HPRT is a purine salvage enzyme that converts purine bases and PRPP to GMP and IMP, which are precursors of the essential nucleotide GTP. HPRT activity was previously found to be inhibited by (p)ppGpp in several bacteria including Bacillus subtilis. To examine the molecular determinants underlying (p)ppGpp regulation of HPRT, we turned to Hpt-1 from the pathogenic bacterium B. anthracis, which pppGpp competitively inhibits similarly to B. subtilis HPRT. We crystallized Hpt-1 with and without ppGpp, and for comparison, we also crystallized Hpt-1 with its two substrates, PRPP and the non-reactive guanine analog 9-deazaguanine.

We next interrogated the effect of (p)ppGpp on the oligomeric state of HPRT using the protein crosslinker dimethyl adipimidate (DMA). Crosslinked apo HPRT was resolved by SDS–PAGE as bands corresponding to monomers, dimers, trimers, or tetramers (lane 2). All but the tetramer is likely formed by incomplete crosslinking, since dynamic light scattering showed apo B. anthracis Hpt-1 to be a homogeneous population with a hydrodynamic radius (RH) consistent with a tetramer in solution.

>SNAMMNQDIEKVLISEEQIQEKVLELGAIIAEDYKNTVPLAIGVLKGAMPFMADLLKRTDTYLEMDFMAVSSYGHSTVSTGEVKILKDLDTSVEGRDILIVEDIIDSGLTLSYLVDLFKYRKAKSVKIVTLLDKPTGRKVDLKADYVGFTVPHEFVVGYGLDYKEQYRNLPYVGVLKPSVYSN[4x]> MTEAMVHVDEASAVRRGVDFLLDRREADGRWVDYDLLGPSDDWITAYVAGVLVQLPHEAAGRAGRAAMDLLVPEQHDNGGWNYSEVAPEDADSTGWVLRLAELLGRSGEPWARPGWEFLARHVHDDGLVSTYVPDLAKAAFDRYPVVPSWDGWCGGHVCVTAAVAGLAGLPRREH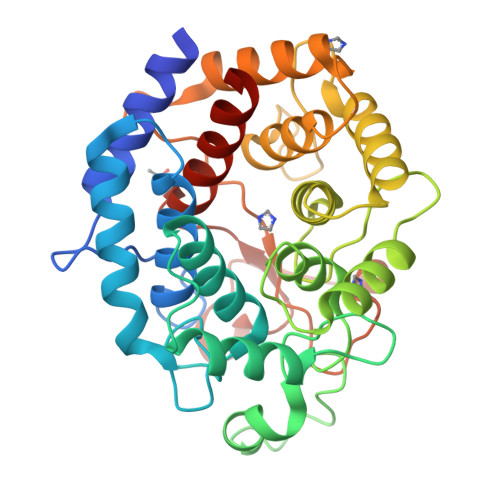VVNGLLRAQRPTGEWPAYWWIDPELSTALAVESLATVPGTEPARAAAARWAAGRIGADGAVTTHLHPEGSPFATALALRAVAQGEPGFGDAQIRAAAGWLTRHQRPDGSWTPSARLRMVLPWETDPDSYEDWTFDGVGRACLGTIARDTFGLHTTATVLQALRTAATRTGA> L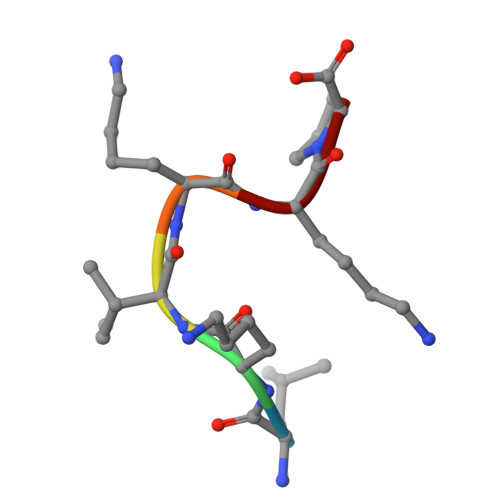KIKKP>[8x]SNAMGKKIRTEEVDHLFEAIL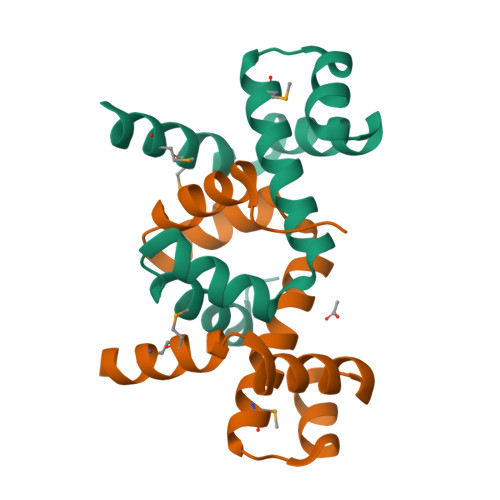CLKNKEECYTFFEDVCTINELLSLSQRFEVAKMLTDKRTYLDISEKTGASTATISRVNRSLNYGNDGYEMVFSRMKEKETAGKTEE>GPMSVPTDGAVTTSQIPA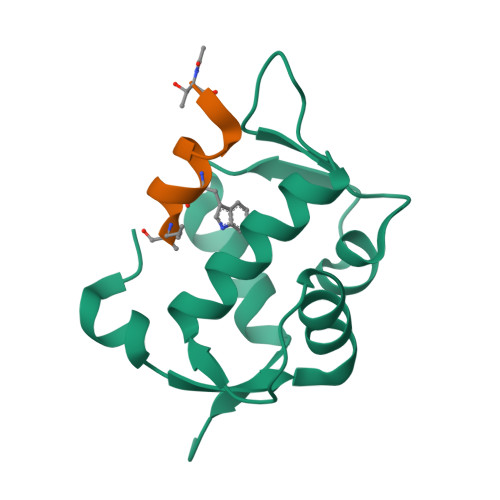SEQETLVRPKPLLLKLLKSVGAQKDTYTMKEVLFYLGQYIATKRLYDEKQQHIVYCSNDLLGDLFGVPSFSVKEHRKIYTMIYRNLVVVNQQESSDSGTSVSEN[2x];>[2x]TSFXEYWALLLX>[4x]MRKLNPALEFRDFIQVLKDEDDLIEITEEIDPNLEVGAIMRKAYESHLPAPLFKNLKGASKDLFSILGCPAGLRSKEKGDHGRIAHHLGLDPKTTIKEIIDYLLECKEKEPLPPITVPVSSAPCKTHILSEEKIHLQSLPTPYLHVSDGGKYLQTYGMWILQTPDKKWTNWSIAAGMVVDDKHITGLVIKPQHIRQIADSWAAIGKANEIPFALCFGVPPAA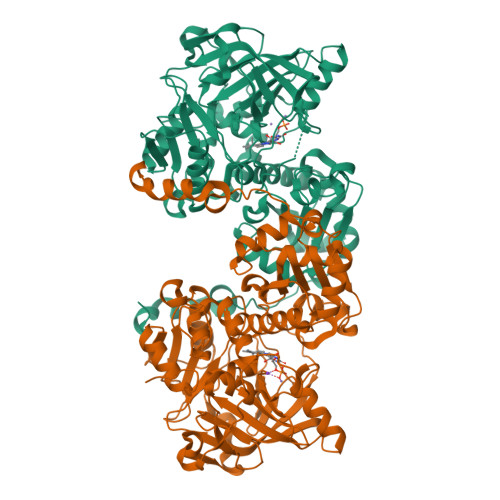ILVSSMPIPEGVSESDYVGAILGESVPVVKCETNDLMVPATSEMVFEGTLSLTDTHLEGPFGEMHGYVFKSQGHPCPLYTVKAMSYRDNAILPVSNPGLCTDETHTLIGSLVATEAKELAIESGLPILDAFMPYEAQALWLILKVDLKGLQALKTTPEEFCKKVGDIYFRTKVGFIVHEIILVADDIDIFNFKEVIWAYVTRHTPVADQMAFDDVTSFPLAPFVSQSSRSKTMKGGKCVTNCIFRQQYERSFDYITCNFEKGYPKGLVDKVNENWKRYGYKHHHHHH>MGLPPLLSLPSNSAPRSLGRVETPPEVVDFMVSLAEAPRGGRVLEPACAHGPFLRAFREAHGTGYRFVGVEIDPKALDLPPWAEGILADFLLWEPGEAFDLILGNPPYGIVGEASKYPIHVFKAVKDLYKKAFSTWKGKYNLYGAFLEKAVRLLKPGGVLVFVVPATWLVLEDFALLREFLAREGKTSVYYLGEVFPQKKVSAVVIRFQKSGKGLSLWDTQESESGFTPILWAEYPHWEGEIIRFETEETRKLEISGMPLGDLFHIRFAARSPEFKKHPAVRKEPGPGLVPVLTGRNL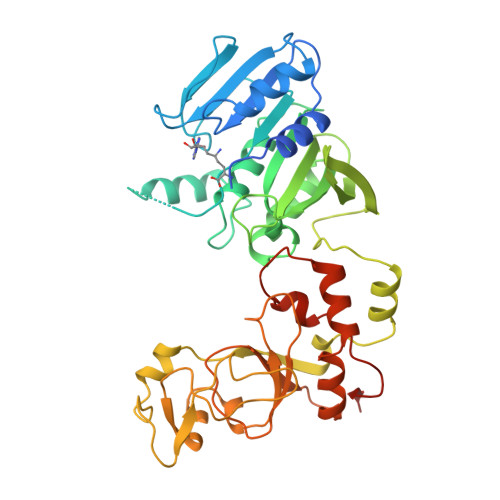KPGWVDYEKNHSGLWMPKERAKELRDFYATPHLVVAHTKGTRVVAAWDERAYPWREEFHLLPKEGVRLDPSSLVQWLNSEAMQKHVRTLYRDFVPHLTLRMLERLPVRREYGFHTSPESARNF[2x]>MSKNEKDEIKIVKYPDPILRRRSEEVTNFDDNLKRVVRKMFDIMYESKGIGLSAPQVNISKRIIVWNALYEKRKEENERIFINPSIVEQSLVKLKLIEGCLSFPGIEGKVERPSIVSISYYDINGYKHLKILKGIHSRIFQHEFDHLNGTLFID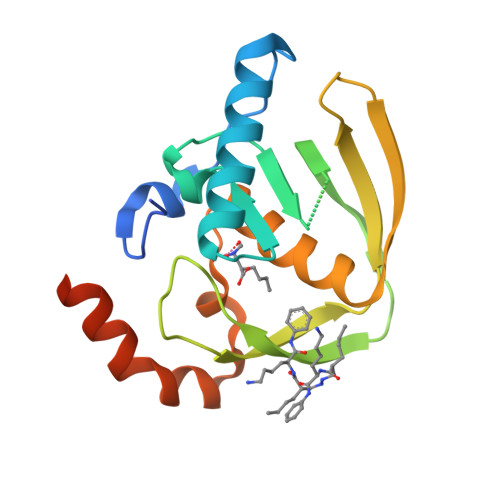KMTQVDKKKVRPKLNELIRDYKATHSLEHHHHHH[2x]> LTLGLAPALSTHSSGVSTQSVDLSQIKRGDEIQ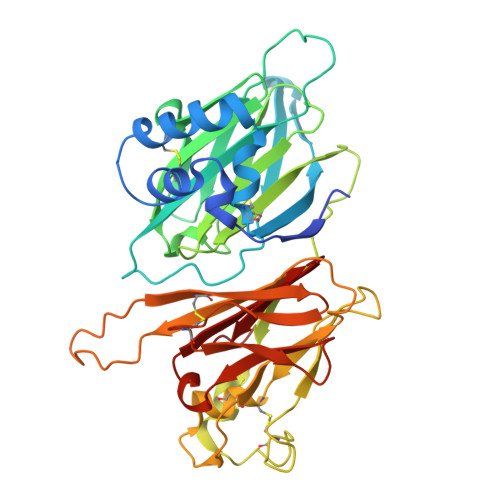AHCLTPAETEVTECAGILKDVLSKNLHELQGLCNVKNKMGVPWVSVEELGQEIITGRLPFPSVGGTPVNDLVRVLVVAESNTPEETPEEEFYAYVELQTELYTFGLSDDNVVFTSDYMTVWMIDIPKSYVDVGMLTRATFLEQWPGAKVTVMIPYSSTFTWCGELGAISEESAPQPSLSARSPVCKNSARYSTSKFCEVDGCTAETGMEKMSLLTPFGGPPQQAKMNTCPCYYKYSVSPLPAMDHLILADLAGLDSLTSPVYVMAAYFDSTHENPVRPSSKLYHCALQMTSHDGVWTSTSSEQCPIRLVEGQSQNVLQVRVAPTSMPNLVGVSLMLEGQQYRLEYFGDH>SEKLTFKTDLEKLEREKAAQIGVAIVDPQGEIVAGHRMAQRFAMCSTFKFPLAALVFERIDSGTERGDRKLSYGPDMIVEWSPATERFLASGHMTVLEAAQAAVQLSDNGATNLLLREIGGPAAMTQYFRKIGDSVSRLDRKEPEMNDNTPGDLRDTTTPIAMARTVAKVLYGGALTSTSTHTIERWLI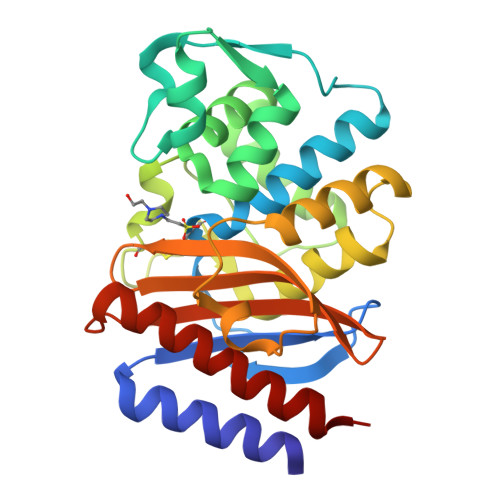GNQTGDATLRAGFPKDWVVGEKTGTCANGGRNDIGFFKAQERDYAVAVYTTAPKLSAVERDELVASVGQVITQLILSTDK[2x]> AATTQIGEIVKTVANTVESEIKAELGVIPSLNAVETGATSNTEPEEAIQTRTVINMHGTAECLVENFLGRSALVCMRSFEYKNHSTSTSSIQKNFFIWTLNTRELVQIRRKMELFTYLRFDTEITIVPTLRLFSSSNVSFSGLPNLTLQAMYVPTGARKPSSQDSFEWQSACNPSVFFKINDPPARLTIPFMSINSAYANFYDGFAGFEKKATVLYGINPANTMGNLCLRVVNSYQPVQYTLTVRVYMKPKHIKAWAPRAPRTMPYTNILN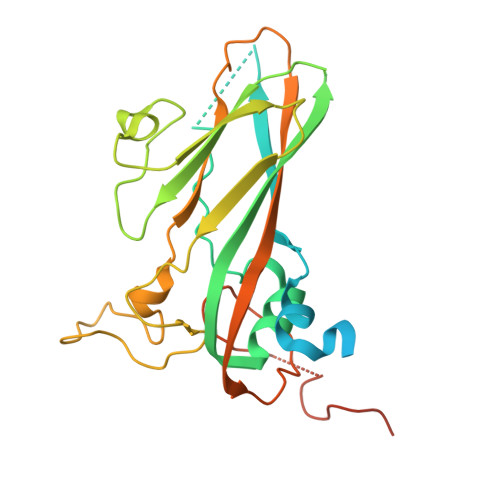NNYAGRSAAPNAPTAIVSHRSTIKTMPNDINLTTA>[2x]MSLEKQIESYYQEIAQLIIDMIPEEWAEVRF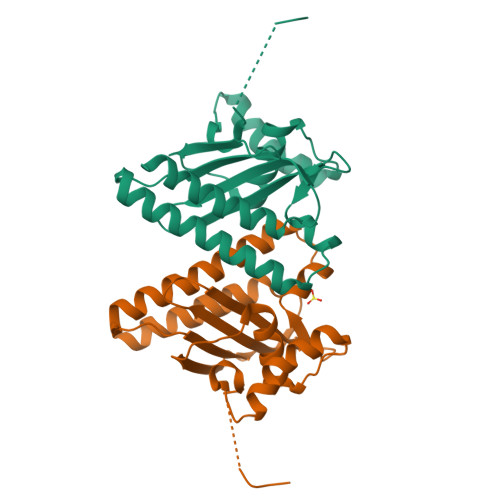YAQEDHDGWKIFFFHYLSASSDEWTKDIDIRDVIKVPQDEFMEKYNELSFCISDFRKDYAEAFGEPWMSFQMTFYASGKFNIDFYYDKNPFDTFLTRLAWQYEHFGTIPEDSFYKETLNEYLEEKAQGKRYPFLEPLKEEEGHHHHHH>[4x]MAKVTELGYLGLSVSNLDAWRDYAAG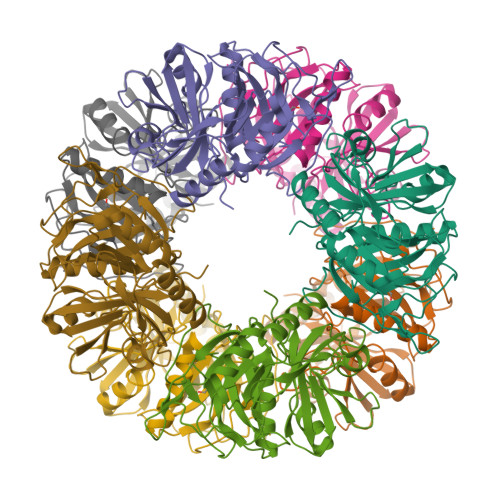IMGMQVVDDGEDDRIYLRMDRWHHRIVLHADGSDDLAYIGWRVAGPVELDELAEQLKNAGIPFEVASDADAAERRVLGLVKLHDPGGNPTEIFYGPQVDTSSPFHPGRPMFGKFVTEGQGLGHIIIREDDVEEATRFYRLLGLEGAVEYKFALPNGAVGTPVFMHCNDRHHSLAFGVGPMDKRINHLMIEYTHLDDLGYAHDLVRQQKIDVTLQIGKHSNDEALTFYCANPSGWLWEPGWGSRPAPAQQEHYLRDIFGHDNEVEGYGLDIPLKGLDIPA> MILANVFCLFFFLDETLRSLASPSSLQGPELHGWRPPVDCVRANELCAAESNCSSRYRTLRQCLAGRDRNTMLANKECQAALEVLQESPLYDCRCKRGMKKELQCLQIYWSIHLGLTEGEEFYEASPYEPVTSRLSDIFRLASIFSGTGADPVVSAKSNHCLDAAKACNLNDNCKKLRSSYISICNREISPTERCNRRKCHKALRQFFDRVPSEYTYRMLFCSCQDQACAERRRQTILPSCSYEDKEKPNCLDLRGVCRTDHLCRSRLADFHANCRASYQTVTSCPADNYQACLGSYAGMIGFDMTPNYVDSSPTGIVVSPWCSCRGSGNMEEECEKFLRDFTENPCLRNAIQAFGNGTDVNVSPKGPSFQATQAPRVEKTPSLPDDLSDSTSLGTSVITTCTSVQEQGLKANNSKELSMCFTELTTNIIPGSNKVIKP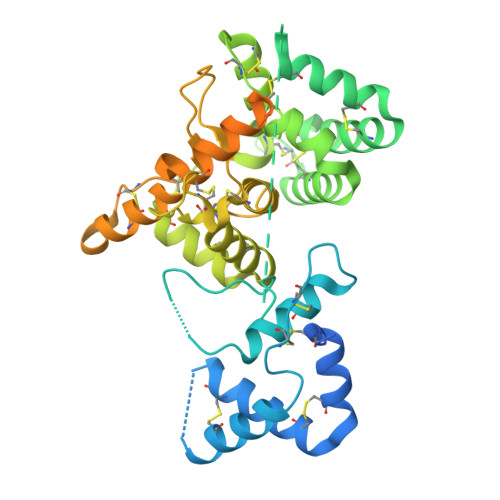NSGPSRARPSAALTVLSVL> AYDVLIVGS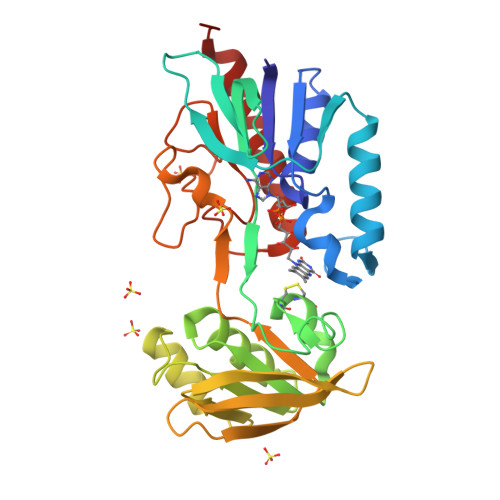GPAGAAAAIYSARKGIRTGLMGERFGGQILDTVDIENYISVPKTEGQKLAGALKVHVDEYDVDVIDSQSASKLIPAAVEGGLHQIETASGAVLKARSIIVATGAKWRNMNVPGEDQYRTKGVTYCPHCDGPLFKGKRVAVIGGGNSGVEAAIDLAGIVEHVTLLEFAPEMKADQVLQDKLRSLKNVDIILNAQTTEVKGDGSKVVGLEYRDRVSGDIHNIELAGIFVQIGLLPNTNWLEGAVERNRMGEIIIDAKCETNVKGVFAAGDCTTVPYKQIIIATGEGAKASLSAFDYLIRTKTA>[2x]SPRMDDHGLKEICLDHLYRGCQQVNCNKNHFHLPYRWQLFILPTWMDFQDMEYIER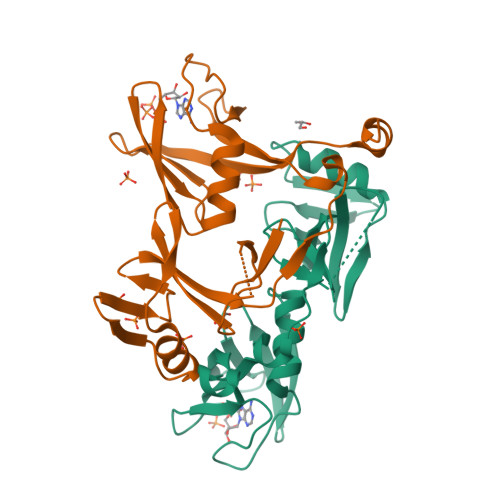AYCDPQIEIIVIEKHRINFKKMTCDSYPIRRLSTPSFVEKTLNSVFTTKWLWYWRNELNEYTQYGHESPSHTSSEINSAYLESFFHSCPRGVLQFHAGSQNYELSFQGMIQTNIASKTQRHVVRRPVFVSSKDVEQKRRGPD>[6x]AEIYNKDGNKVDLYGKAVGLHYFSKGNGENSYGGNGDMTYARLGFKGETQINSDLTGYGQWEYNFQGNNSEGADAQTGNKTRLAFAGLKYADVGSFDYGRNYGVVYDALGYTDMLPEFGGDTAYSDDFFVGRVGGVATYRNSNFFGLVDGLNFAVQYLGKNERDTARR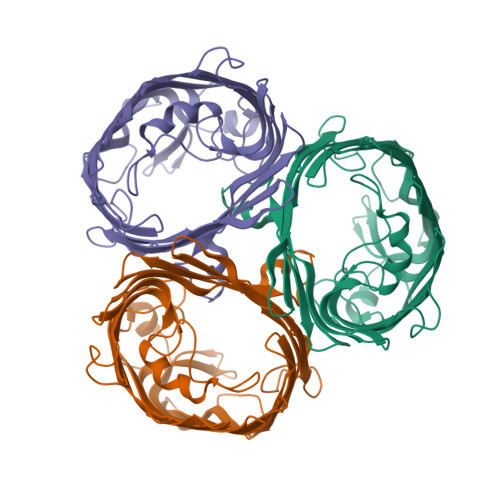SNGDGVGGSISYEYEGFGIVGAYGAADRTNLQEAQPLGNGKKAEQWATGLKYDANNIYLAANYGETRNATPITNKFTNTSGFANKTQDVLLVAQYQFDFGLRPSIAYTKSKAKDVEGIGDVDLVNYFEVGATYYFNKNMSTYVDYIINQIDSDNKLGVGSDDTVAVGIVYQF> MWHYTSINNDTRVALDPKPNQIRTITKPNTVPQLGTDYLYTFNSQRRSHTLRLLGPFQYFNFSETDRGHPLFRLPLKYPSKAIPADELIDNLHSWMRSVHLLHVRSEDNTLRYNWMLGVYARSTNYTTPVGQLVVNAPAILNYSNPQDAFNSVFVALGIDYIDIPITNSNIFDDSSTPYNVRIWHAPTMTEVNHILALMRKSTLVSTHSSWHWNVLHTFHYRSESDMIDHFAAKILEDWRQKEKLDKGALVEADRVIQRLIPLSSSTYVQRLAAIGALYPNEFTENVLDLSRLSTALLQLSDTYYQHANDQLRRLYRRMYNDSRTLYMTQRHQELLLAQITADPNILLYPYTYIFTTIPTSMNYISNTGQGRIKHSLTVTGATEHDTVADIVLGQTGEDVITISMVEPMSIAVEDMYGYVLDTPTRDIWPADEQIEQKGDAVALYDTKTSRALGMFNNTVRIDDLLSPLLSLVYRTYIKGDTMTMTQGSLDHLTLCAAVDSDITFVGNRMIAPLPEGYIPKPMHRNNSTMKMLSLYVALKKLENFATNSYLMAPDTSIILLGAEREPAVNILRRFNRNVSNVRIIGMGDRAVEPNIRVRVPFPIDKNISADFIICDINSYEDQSFESMFSETISVVTTCASAATRALVKINHPSEYMINSVIERLSQLGGVFYHTALLKTASQNPYSYETYIYITPIAAAVRFPFYSNSAMINRYMTAVADDEMPIIPSIHTVIKGHSNTYSPGLFCGCVDVQSAPLALSQLKSYCSEATTWRVDSDDNLVNIIARIDPARIALEFRTRSNTSAYHEYQRYVPNGLGFKVRKTREFRYMHREVTFIHKLMMYALIREQISLTENMTQVVSIGGRNLADISVVPLNMKYVVIDPATRIETLTQEKKNIEVQSRPFQFDAANMDLENNSIYLFIAVIMNEPNGAATPARMQMDKIRNVATAMLTRTNCVAYISFYEAGIITRLDQSTAHKTIRVEEGRLKVANYVPVDTLVEADVTLMLRDIGITHEIIRPSTPELIDACSNYGIRLGSTGGAVLDVFNHYSPVIKLVRS;>[2x]MHSTNNNSNKRNNEEKHKQPEIDSSANNGEGTSGTRAQTVGDTATEAGVRNETEAGASTRRQTDGTGLSGTNAKIATASSARQADVEKPADVTFTIENVDDVGIMQQKKPPTVVQSRTDVFNEQFANEALHPTTKVIFNGLDVNTEVQPLSDDFKQISDPKGYLTYSVKYEDQFTKKDKLRASEADDRIVGPTVNLFKYGAAVVNIDLNRDFFDTATGIDLTKGIPLVQDLLVPIGVTAGAEQSAEYVSGLLMVLFKVMTDNRLVIVGETTTPMSNTLSTVVNNVLRTTYHNNVGVNPALLRDFTQVNWLNRDITNMLQQAGTKYGLGLTETRLDYVRLVKTIVGHALNIDHFAASVLNINLRALMEANVTADDRIKALQAHSMISTQFHGPNQGALRPELAFDHDHIIRCLMLAAANYPRLEGIIVQINTGYVASANVIRPVSEKRYFPENLEQNQSAARLVSAVKARASEADISSIHLAIAREVSPMFNVHELKKIAESFEDPSSIVVVLEFILFALFFPTEFNRIKGDIQNVLLLFFSRWYPVEYGIFVQRGATYTINAAGEFEFSGRNEKWDQALYLSEHFPALFSDVPLAGANTIIAIMRLFTPQGFLRTDDLAIAANFPRASRNPQTYIPYTNQRGTVTNEFASRFRTIVATLANVVNERAVQDDMQKATRSCTKQWLRHLETQFDNIAVAHTDHLSVVYATMSNFMLNFTNNFSGNHATFKPDQYVITSPEGSYKPIIERQGETVDGLTIIDTSIVWPILCQCTYPLVRQSGKGVDAVSIMEEIVYPDPSTTLSQSLSVAQVLSKLTLPDAFINMILSGGDSVVMRTYQTEADDDLDEGIRMTTYDQYLSHIRERLHITNVPDPIYITGASTPDQIAASVQA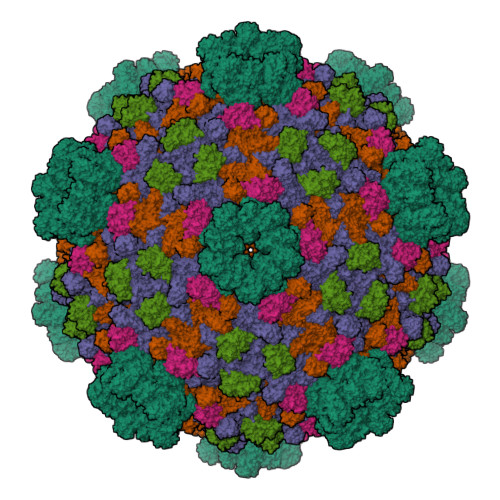THVAVVLYQSGVINGPASTYLRENEVLVVMPDYYDVVSRFANANLQMNNNRYHESVLEIADIFDQADFIQTSDAVRQLRALMPTLSTSQIRHAIERIAQITDVDSTDYGKLTLRFLGTLTRSLKMQNAQIRRIRPDGTVLRYDDQIDIEAFRWSRYFLDELQLRRLSVGLRLITNPRIARRFNGVRIMYLTDDDPDPDFVPDVPEGYVAVQYAHRLFSSSLANKRNRVTYTHPPTGMAYPSPTGRPHVHMTINERAGMSKLVADNIIASVIKSNWVVDILDIEYTAEVMTPSEGYTQHVDAESIMTAPKGKLFHLQFMDGLLRPEPSAFDPPASGEDMRLIYPLQPISVARSMRAIVNHNEVDRPRGAVAPSSYEMDTGTLSRNGDLLYSPVANGQVGIPKLEVDHISFSNVVSMMTANIRTGDDMAVERVNPDDVRAINIRNA;>[2x]MLQQPTGGYTTLEQFAFTIRNDGTNATPTQFLQLLSYEATENELVKKTIPTPETHLPSARNVPGNVYIEDAITQALFGISAQNVNAHGYFSRLSALALPNTSARLGLDGVIYNSETINIPFYDPAAVANFAATYAKLGNASTPRYRADMIDIYAHVGLELAGTDAERAAGVMPVKRAKFDSWEGSLISLSRDVVNWKILAFLIDLCSLEGEALRAFKTRNRDVFRMMLFIMSTAVAANVVNRKVTKRVDRVLEYIGVNSMRTAGRTATITYDLSRHEFAAKFLQLTFTRWNAASAMIRSMPDMHTPRTSITPAGENALVRHNRYMTENFKGLSPIALAQKKHEMMLHTHEIHSMDIDGSIKNMVERETVNKMNEIDAMNTAPWTEEFAEVEPTTVYERHQIGTDPEQTQLISQDAAVIVHQASSDVDENEYGNSVSELTIDTQSDSVL> SDAHDEETFEEFTARYEKEFDEAYDLFEVQRVLNNCFSYDLVPAPAVIEKALRAARRVNDLPTAIRVFEALKYKVENEDQYKAYLDELK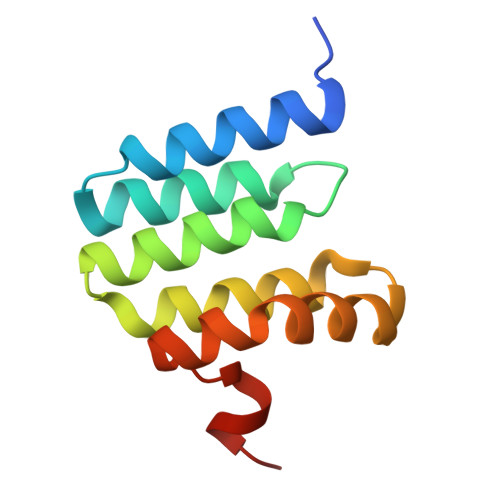DVRQELGVPLKEELFPSSS>MNTKIKVAIVG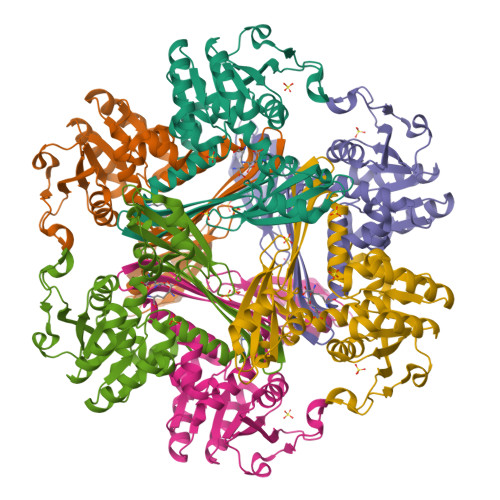YGNIGRFALEAVQAAQDFELVGVVRRDINNVPEELQNITVTNDIKTLGDVDVALLCSPTRAIKELAKSILSLGINTVDSFDVHSEIVSLKTELDDVAKKHDRVAVISAGWDPGSDSIVRTLMLAMAPKGITYTNFGPGMSMGHSVAAKAIEGVKDALSMTIPLGTGVHRRMVYVELEAGANFNQVEQAIKADSYFSSDETHVKQVDSVDSLKDVGHGVHMTHKGVSGKTHNQLFEYSMRINNPALTSQFMVSAARASMKQRAGAYTVIEIPPVDFLAGDLNTLIAKLV[4x]>[2x]GFKQDIATLRGDLRTYAQDIFLAFLNKYPDEKRNFKNYVGKSDQELKSMAKFGDHTEKVFNLMMEVADRATDCVPLASDASTLVQMKQHSGLTTGN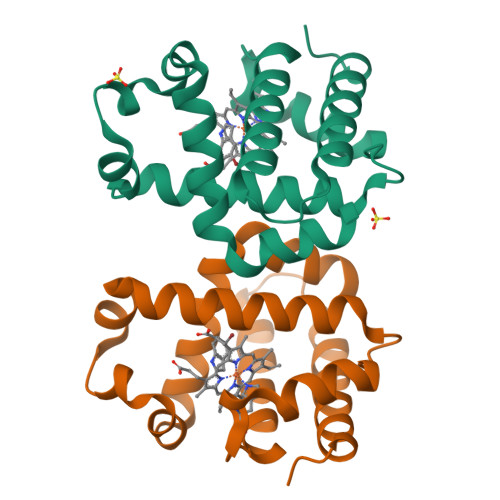FEKLFVALVEYMRASGQSFDSQSWDRFGKNLVSALSSAGMK>MSESAKVWLVTGASSGFGRAIAEAAVAAGDTVIGTARRTEALDDLVAAYPDRAEAISLDVTDGERIDVVAADVLARYGRVDVLVNNAGRTQVGAFEETTERELRDLFELHVFGPARLTRALLPQMRERGSGSVVNISSFGGQLSFAGFSAYSATKAALEQLSEGLADEVAPFGIKVLIVEPGAFRTNLFGKGAAYFSEENPAYAEKVGPTRQLVQGSD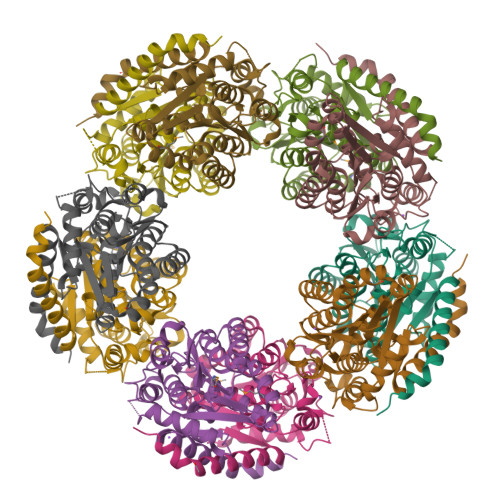GSQPGDPAKAAAAIRLALDTEKTPLRLALGGDAVDFLTGHLDSVRAELTEWEKVSRGTDFDTE[10x]> MAKKTPPVYPVTVPFLGHIVQFGKNPLEFMQRCKRDLKSGVFTISIGGQRVTIVGDPHEHSRFFSPRNEILSPREVYTIMTPVFGEGVAYAAPYPRMREQLNFLAEELTIAKFQNFVPAIQHEVRKFMAENWKEDEGVINLLEDCGAMIINTACQCLFGEDLRKRLNARHFAQLLSKMESSLIPAAVFMPWLLRLPLPQSARCREARAELQKILGEIIV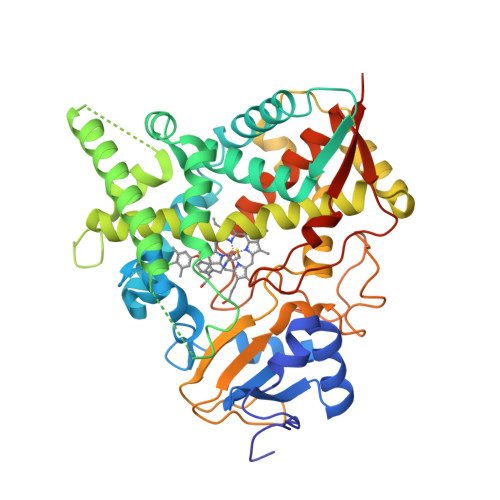AREKEEASKDNNTSDLLGGLLKAVYRDGTRMSLHEVCGMIVAAMFAGQHTSTITTSWSMLHLMHPKNKKWLDKLHKEIDEFPAQLNYDNVMDEMPFAERCVRESIRRDPPLLMVMRMVKAEVKVGSYVVPKGDIIACSPLLSHHDEEAFPNPRLWDPERDEKVDGAFIGFGAGVHKCIGQKFALLQVKTILATAFREYDFQLLRDEVPDPDYHTMVVGPTLNQCLVKYTRKKKLPSHHHHHH>GMRKPKITVIGGGTGSPVILKSLREKDVEIAAIVTVADDGGSSGELRKNMQQLTPPGDLRNVLVAMSDMPKFYEKVFQYRFSEDAGAFAGHPLGNLIIAGLSEMQGSTYNAMQLLSKFFHTTGKIYPSSDHPLTLHAVFQDGTEVAGESHIVDHRGIIDNVYVTNALNDDTPLASRRVVQTILESDMIVLGPGSLFT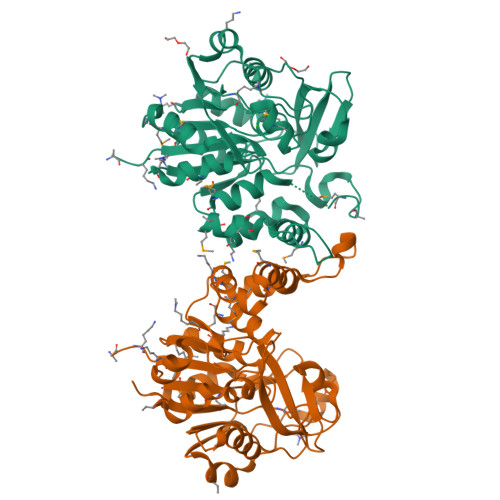SILPNIVIKEIGRALLETKAEIAYVCNIMTQRGETEHFTDSDHVEVLHRHLGRPFIDTVLVNIEKVPQEYMNSNRFDEYLVQVEHDFVGLCKQVSRVISSNFLRLENGGAFHDGDLIVDELMRIIQVKK[2x]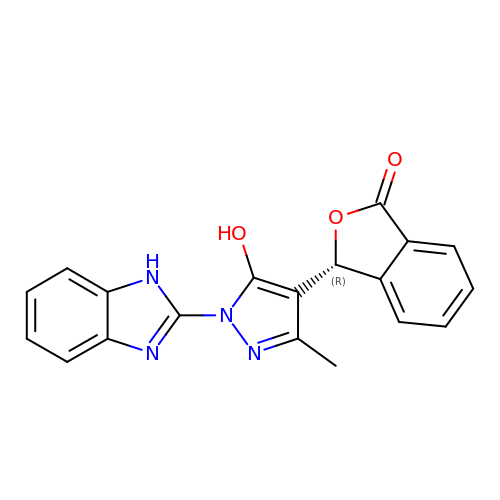(3R)-3-[1-(1H-benzimidazol-2-yl)-5-hydroxy-3-methyl-1H-pyrazol-4-yl]-2-benzofuran-1(3H)-one | C19 H14 N4 O3 | JRMYHMGBFVARON-MRXNPFEDSA-N>PKLVLVRHGQSEWNEKNLFTGWVDVKLSAKGQQEAARAGELLKEKKVYPDVLYTSKLSRAIQTANIALEKADRLWIPVNRSWRLNERHYGDLQGKDKAETLKKFGEEKFNTYRRSFDVPPPPIDASSPFSQKGDERYKYVDPNVLPETESLALVIDRLLPYWQDVIAKDLLSGKTVMIA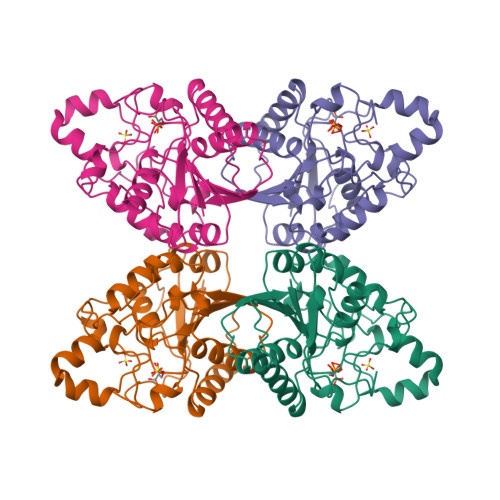AHGNSLRGLVKHLEGISDADIAKLNIPTGIPLVFELDENLKPSKPSYYLDPEAAAAGAAAV[2x]> ASMQKLINSVQNYAWGSKTALTELYGIANPQQQPMAELWMGAHPKSSSRITTANGETVSLRDAIEKNKTAMLGEAVANRFGELPFLFKVLCAAQPLSIQVHPNKRNSEIGFAKEN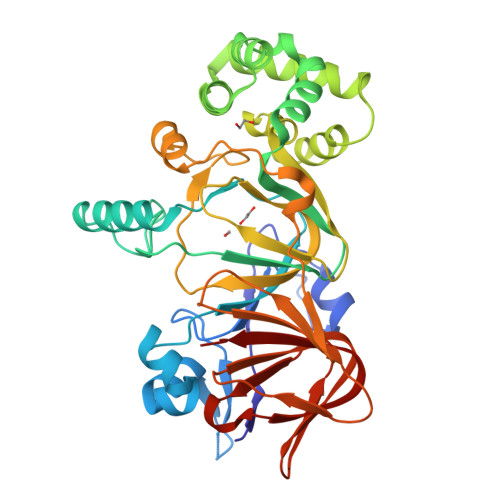AAGIPMDAAERNYKDPNHKPHLVFALTPFLAMNAFREFSDIVSLLQPVAGAHSAIAHFLQVPNAERLSQLFASLLNMQGEEKSRALAVLKAALNSQQGEPWQTIRVISEYYPDDSGLFSPLLLNVVKLNPGEAMFLFAETPHAYLQGVALEVMANSDNVLRAGLTPKYIDIPELVANVKFEPKPAGELLTAPVKSGAELDFPIPVDDFAFSLHDLALQETSIGQHSAAILFCVEGEAVLRKDEQRLVLKPGESAFIGADESPVNASGTGRLARVYNKL>[2x]MAEEGTRSEAADAATQARQLPDSRNIFVSHRFPERQVDLGEVVMNFAEAGSPDNPALLLLPEQTGSWWSYEPVMGLLAENFHVFAVDIRGQGRSTWTPRRYSLDNFGNDLVRFIALVIKRPVVVAGNSSGGLLAAWLSAYAMPGQIRAALCEDAPFFASELVPAYGHSVLQAAGPAFELYRDFLGDQWSIGDWKGFVEAAKASPAKAMQLFPTPDEAPQNLKEYDPEWGRAFFE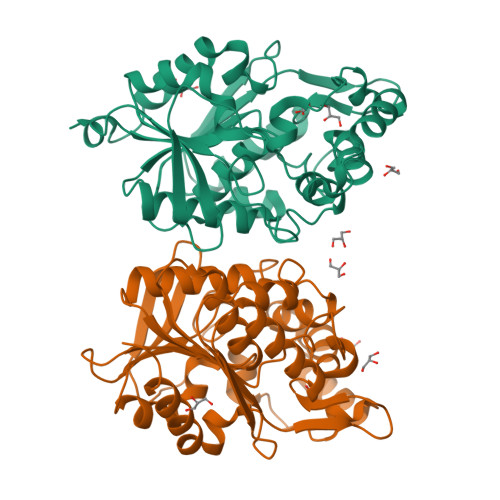GTVALHCPHDRMLSQVKTPILITHHARTIDPETGELLGALSDLQAEHAQDIIRSAGVRVDYQSHPDALHMMHLFDPARYAEILTSWSATLPANDHHHH(2M)-2-(2-methoxyphenyl)-1,3,4-oxadiazole 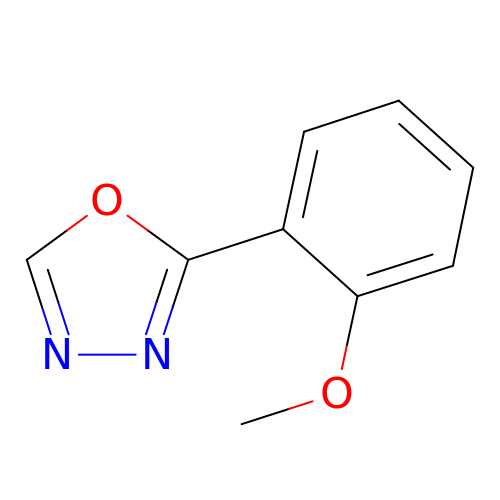| C9 H8 N2 O2 | CMZBFAJLBDAJMC-UHFFFAOYSA-N>HHNKVRTCWNEGRPALAGWLQLPGTLHAEALARLDYDAVVIDMQHSPIDFGQVAPMLIAIELGGAEPFVRTQVNDPSDIMKLLDAGAYGIIAPMVNTRAEAQTLASALHYSPRGLRSFGPRRPSLRYGSGYLAQASETVVGLAMIETREALANIDEILSVDGIDGVFIGPTDLALDLGHAPLVDTEEAEVVSAIAHVRERAHAAGKRVGIFCGSGGFARVKLAEGF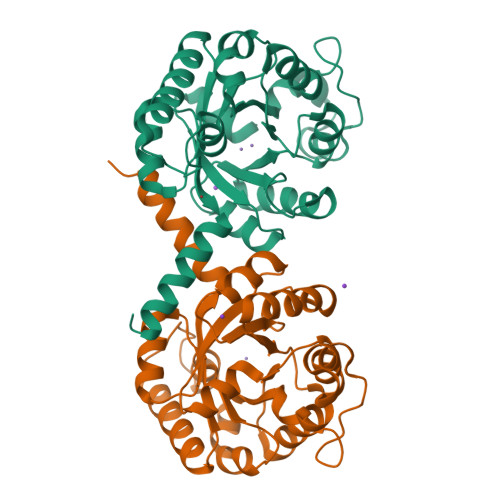DFVTAAPDLAMLSAAARQVIADARAL[2x]(2S)-4-(2,5-difluorophenyl)-N-[(3R,4S)-3-fluoro-1-methylpiperidin-4-yl]-2-(hydroxymethyl)-N-methyl-2-phenyl-2,5-dihydro-1H-pyrrole-1-carboxamide | C25 H28 F3 N3 O2 | 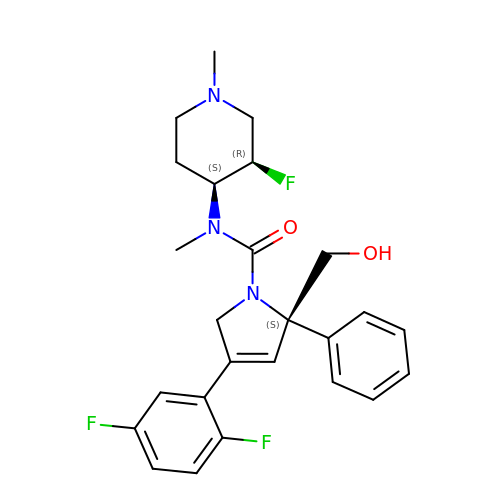MYBGWENAVMIGMM-GIFXNVAJSA-N>[2x]GSKVEDPKDFPSELLSFLSHAVFSNRTLACFAIYTTKEKAALLYKKIMEKYSVTFISRHNSYNHNILFFLTPHRHRVSAINNYAQKLCTFSF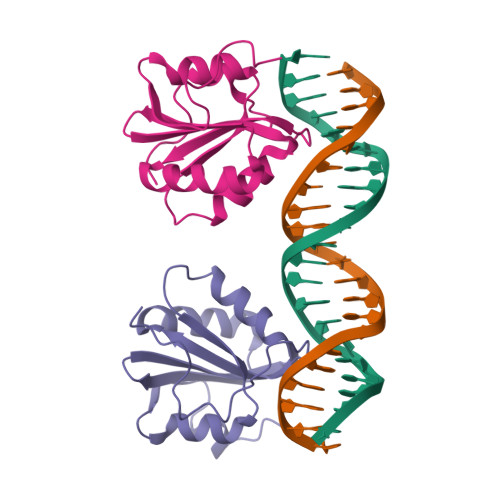LICKGVNKEYLMYSALTRDPFSVIEESLPGGLKEHDFNPESS>[2x]MPI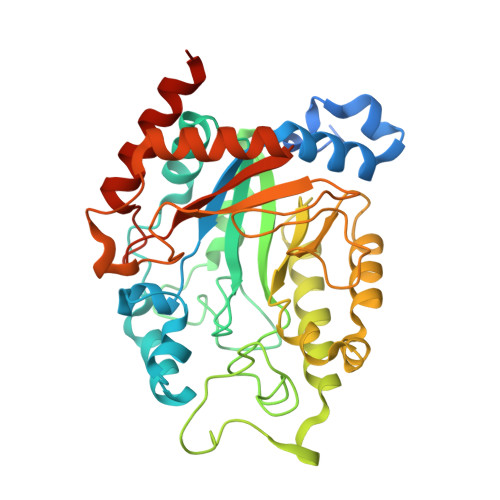QNINRRSLLCSGAATTAALAVSPSVFGDSAVPSYLKDYAALYKKDPRAAALQYFKEAKFGLFIHYGLYSLLGRGEWVQLQGKIPVREYAKLENDFTAKNFDADFITDMALEAGMKYVNITTRHHDSFCLFESKYTDFTSTNSPAKRDLVAELAEECRKKGLGFYLYYSHGRDWRHPHAPNNGDWGGNARPKYDSPEPFYKYGEDQDLQIYVEFMKNQITELLTNYGPVGGIWLDGVATPASRKGKLHLFETQELYDHIHSLQPQVLVSYKQGLIGTEDFKAPERHFKGTSDVPLEFCDTLQPWKWGYDKSLDGKHKTADQVMEMLSKANKMDANLLLNVGPLPDGSIHPEDVKTLAEVGRKLKAHHHHHH1-(4-methylphenyl)-2-[(1S,2R,5R,8R,8aR)-1,2,8-trihydroxyoctahydroindolizin-5-yl]ethanone 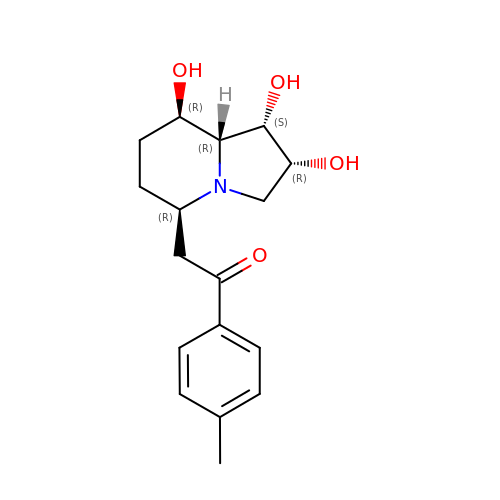| C17 H23 N O4 | APAFVLSHHZZYGV-PVTMVUMOSA-N>GSHMSNTQTVLPFTGLNTPNGVAVDSAGTVYVTDHGNNRVVKLAAGSNTQTVLPFT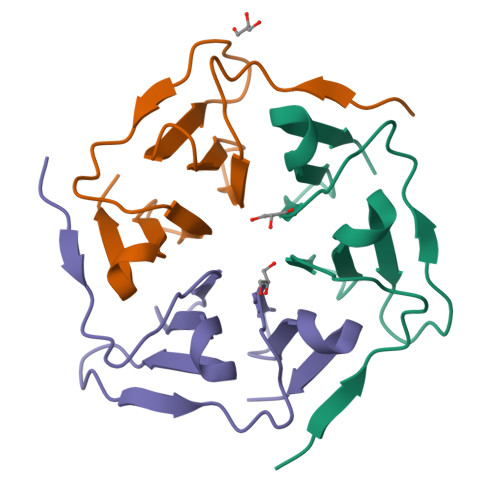GLNTPNGVAVDSAGTVYVTDHGNNRVVKLAAG[3x]>MRLELPVIPLRNTVILPHTTTPVDVGRAKSKRAVEEAMGADRLIFLVAQRDPEVDDPAPDDLYTWGVQAVVKQAMRLPDGTLQVMVEARARAQVTDYIPGPYLRARGEVFSEIFPIDEAVVRVLVEELKEAFEKYVANHKSLRLDRYQLEAVKGTSDPAMLADTIAYHATWTVAEKQEILELTDLEARLKKVLGLLSRDLERFELDKRVAQRVKEQMDTNQREYYLREQMKAIQKELGGEDGLSDLEALRKKIEEVGMPEAVKTKALKELDRLERMQQGSPEATVARTYLDWLTEVPWSKADPEVLDINHTRQVLDEDHYGLKDVKERILEYLAVRQLTQGLDVRNKAPILVLVGPPGVGKTSLGRSIARSMNRKFHRISLGGVRDEAEIRGHRRTYIGAMPGKLIHAMKQVGVI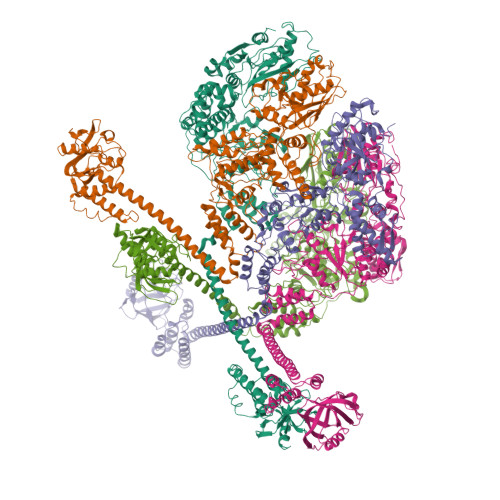NPVILLDEIDKMSSDWRGDPASAMLEVLDPEQNNTFTDHYLDVPYDLSKVFFITTANTLQTIPRPLLDRMEVIEIPGYTNMEKQAIARQYLWPKQVRESGMEGRIEVTDAAILRVISEYTREAGVRGLERELGKIARKGAKFWLEGAWEGLRTIDASDIPTYLGIPRYRPDKAETEPQVGTAQGLAWTPVGGTLLTIEVAAVPGSGKLSLTGQLGEVMKESAQAALTYLRAHTQDYGLPEDFYNKVDLHVHVPDGATPKDGPSAGITMATAIASALSRRPARMDIAMTGEVSLRGKVMPIGGVKEKLLAAHQAGIHKIVLPKDNEAQLEELPKEVLEGLEIKLVEDVGEVLEYLLLPEPTMPPVVQPSDNRQQPGAGA[5x]>[5x]ANPNEAYRHYMKKLSYETDIADLSIDIKKGYEGIIVVDVRDAEAYKECHIPTAISIPGNKINEDTTKRLSKEKVIITYCW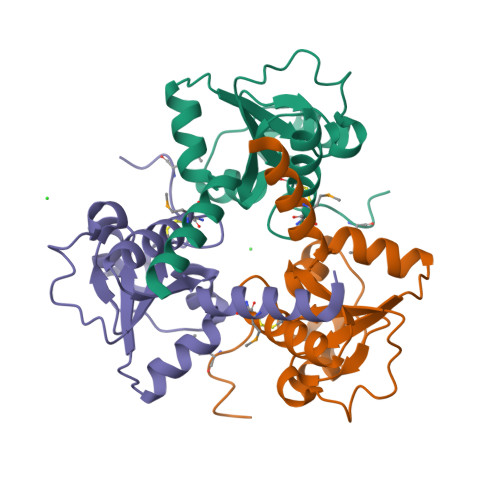GPACNGATKAAAKFAQLGFRVKELIGGIEYWRKENGEVEGTLGAKADLFWNMKKESLEHHHHHH> LPVTVEKPIPVVYDLGNLAAFDSNVLDKNDLDSSNARREEKIKSLTRDNVQLLINQLLSLPMKTT;> SVMTLLQLPDPTTDLPREKPLP;> LVENVKQALFIPGQSCNKNLHDIMVDLSALKKPDMKRFNRKNDIHPFEDMSPLEFFSEKNDCSLMVLMTSSKKRKNNMTFIRTFGYKIYDMIELMVADNFKLLSDFKKLTFTVGLKPMFTFQGAAFDTHPVYKQIKSLFLDFFRGESTDLQDVAGLQHVISMTIQGDFQDGEPLPNVLFRVYKLKSYKSDQGGKRLPRIELVEIGPRLDFKIGRI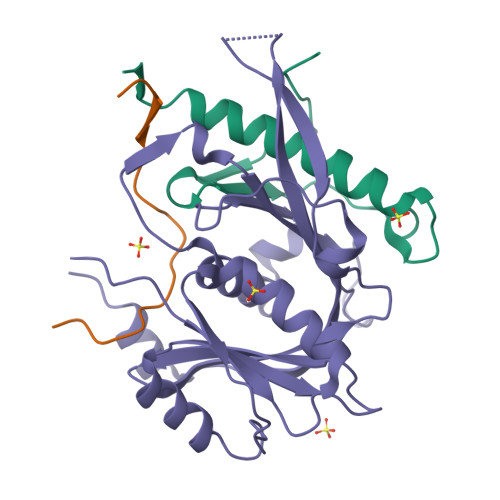HTPSPDMVTEAHKKP1-[(4-methoxyphenyl)methyl]-~{N}-oxidanyl-indole-6-carboxamide | C17 H16 N2 O3 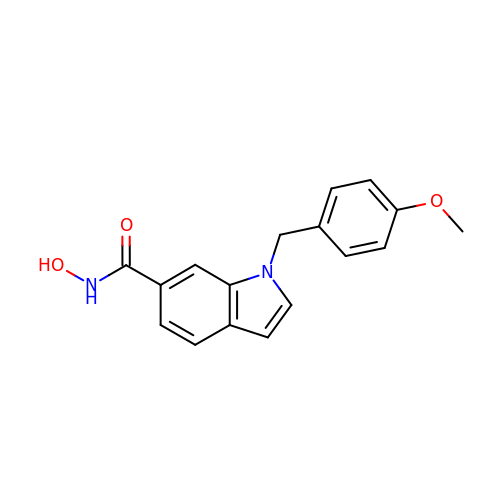| AJRGHIGYPXNABY-UHFFFAOYSA-N3-cyclopropyl-5-methyl-4-phenyl-1,2,4-triazole | C12 H13 N3 | 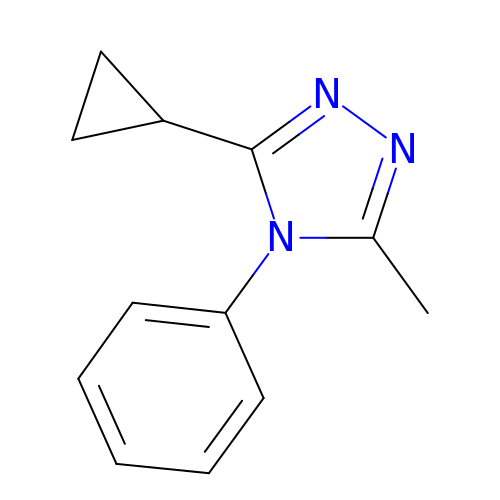NNSGFXSZQIRXDG-UHFFFAOYSA-N>[4x]MATTGTPTADRGDAAATDDPAARFQVQKHSWDGLRSIIHGSRKYSGLIVNKAPHDFQFVQKTDESGPHSHRLYYLGMPYGSRENSLLYSEIPKKVRKEALLLLSWKQMLDHFQATPHHGVYSREEELLRERKRLGVFGITSYDFHSESGLFLFQASNSLFHCRDGGKNGFMVSPMKPLEIKTQCSGPRMDPKICPADPAFFSFINNSDLWVANIETGEERRLTFCHQGLSNVLDDPKSAGVATFVIQEEFDRFTGYWWCPTASWEGSEGLKTLRILYEEVDESEVEVIHVPSPALEERKTDSYRYPRTGSKNPKIALKLAEFQTDSQGKIVSTQEKELVQPFSSLFPKVEYIARAGWTRDGKYAWAMFLDRPQQWLQLVLLPPALFIPSTENEEQRLASARAVPRNVQPYVVYEEVTNVWINVHDIFYPFPQSEGEDELCFLRANECKTGFCHLYKVTAVLKSQGYDWSEPFSPGEDEFKCPIKEEI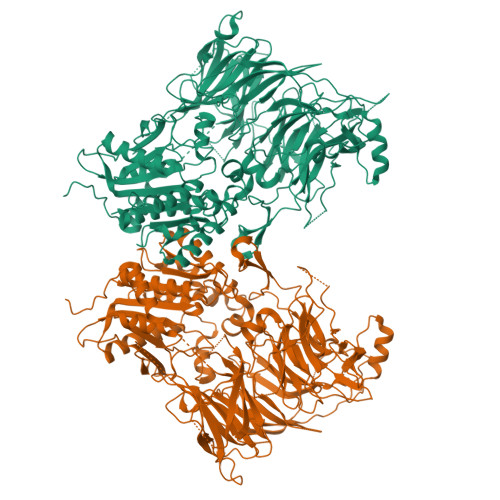ALTSGEWEVLARHGSKIWVNEETKLVYFQGTKDTPLEHHLYVVSYEAAGEIVRLTTPGFSHSCSMSQNFDMFVSHYSSVSTPPCVHVYKLSGPDDDPLHKQPRFWASMMEAASCPPDYVPPEIFHFHTRSDVRLYGMIYKPHALQPGKKHPTVLFVYGGPQVQLVNNSFKGIKYLRLNTLASLGYAVVVIDGRGSCQRGLRFEGALKNQMGQVEIEDQVEGLQFVAEKYGFIDLSRVAIHGWSYGGFLSLMGLIHKPQVFKVAIAGAPVTVWMAYDTGYTERYMDVPENNQHGYEAGSVALHVEKLPNEPNRLLILHGFLDENVHFFHTNFLVSQLIRAGKPYQLQIYPNERHSIRCPESGEHYEVTLLHFLQEYLHHHHHH>[2x]QRCGEQGSNMECPNNLCCSQYGYCGMGGDYCGKGCQNGACWTSKRCGSQAGGATCTNNQCCSQYGYCGFGAEYCGAGCQGGPCRADIKCGSQAGGKLCPNNLCCSQWGFCGLGSEFCGGG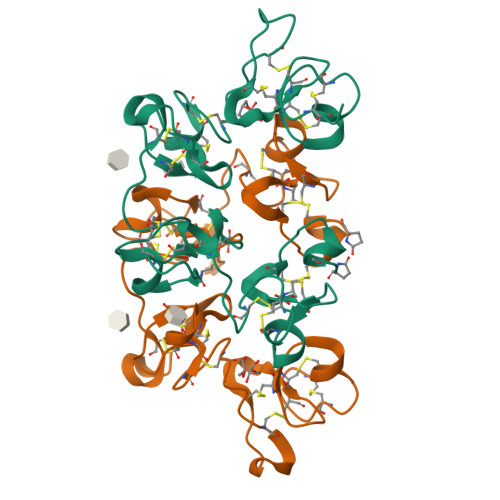CQSGACSTDKPCGKDAGGRVCTNNYCCSKWGSCGIGPGYCGAGCQSGGCDG> GAMDQVQLIKRKDSGRYEIVPIEDPLSFEKGFYAVIRACQLLAQKNDGLILVGLAGPSGAGKTIFTEKILNFMPSIAIINMDNYNDGTRVIDGNFDDPRLTDY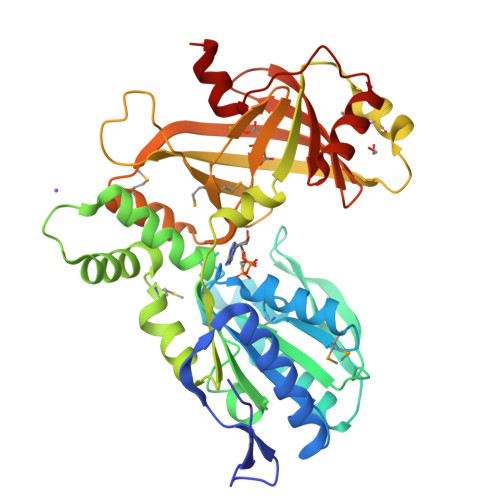DTLLDNIHGLRDGKPVQVPIYDFKSSSRIGYRTLEVPSSRIVILEGIYALSEKLRPLLDLRVSVTGGVHFDLVKRVLRDIQRAGQEPEEIIHQISETVYPMYKAFIEPDLKTAQIKILNKFNPFSGFQNPTYILKSSKAVTPEQMKAALSEDFKERTEETYDIYLLPPGEDPEACQSYLRMRNRDGKYNLMFEEWVTDRPFIISPRITFEVSVRLLGGLMALGYTIATILKRKSHIFDDDKVIVKTDWLEQLNRTYVQVQGKDRTFVKNVADQLGLEGSYVPHTYIEQIQLER We present here a structure-function analysis of one of the best-known HCMV immunevasins, UL16, and its interaction with a cellular ligand for NK cells, MICB. The normal function of MICB is to activate NK cells by engaging the most well-known NK receptor, NKG2D. HCMV-encoded glycoproteins UL16 and UL142 selectively prevent the surface expression of MICB, ULBP1 and ULBP2 (UL16) and MICA (UL142), respectively, through intracellular retention. UL16 is a heavily glycosylated 50 kDa type I transmembrane glycoprotein whose structure could not be predicted from its primary sequence.

In order to elucidate the structural basis for the ability of UL16 to engage highly diverse NKG2D ligands and to compare this promiscuous binding mode to that of NKG2D, we determined the structure of the UL16 ectodomain in complex with the α1α2-platform domain of MICB (MICBpf) at 1.8 Å resolution. In order to obtain soluble and homogeneously glycosylated protein for our structural and surface plasmon resonance (SPR) studies, we expressed the UL16 ectodomain in Chinese hamster ovary (CHO) Lec 3.2.8.1 cells. NK receptors binding to MHC class I or class I-like molecules belong to two structurally distinct families, the Ig superfamily and the C-type lectin superfamily. While NKG2D belongs to the latter group, our structural analysis shows that UL16 assumes an Ig-like fold. We find that UL16, which possesses no structural homology to NKG2D, nevertheless employs a NKG2D-like binding mode to interact with MICB. A set of five predominantly hydrophobic core residues on the UL16 surface precisely mimics a set of five equivalent residues in the central region of the interface used by the structurally unrelated immunoreceptor NKG2D to interact with its ligands. The “rigid adaptation” concept is furthermore supported by the finding that UL16 engages its ligands via a rigid β-sheet, which does not allow for much conformational flexibility. Our structure shows that substitution of Gln169 with arginine, which is present at this position in MICA, would lead to steric clashes with UL16 residues Met59 and Leu161 that would prevent binding. In the UL16-MICBpf complex, Ala162 faces towards Tyr125, a UL16 footprint residue. Taken together, these analyses suggest that some NKG2D ligands apparently bypass intracellular retention by UL16 through alteration of a small number of key residues at strategic locations of their potential UL16 binding interface. To the best of our knowledge, the structure presented here is the first structure of a viral immunoevasin in complex with a stimulatory NK receptor ligand as well as the first reported case of structural mimicry through convergent evolution of a human immunoreceptor by a viral immunoevasin.

>MEPHSLRYNLMVLSQDESVQSGFLAEGHLDGQPFLRYDRQKRRAKPQGQWAEDVLGAETWDTETEDLTENGQDLRRTLTHIKDQKGGLHSLQEIRVCEIHEDSSTRGSRHFYYNGELFLSQNLETQESTVPQSSRAQTLAMNVTNFWKEDAMKTKTHYRAMQADCLQKLQRYLKSGVAIRRTVPPMVNVTCSEVSEGNITVTCRASSFYPRNITLTWRQDGVSLSHNTQQWGDVLPDGNGTYQTWVATRIRQGEEQRFTCYMEHSGNHGTHPVPSGKVLVLQSQRTDFPYVSAAMPCFVIIIILCVPCCKKKTSAAEGP[2x];>VDLGSKSSNSTCRLNVTELASIHPGETWTLHGMCISICYYENVTEDEIIGVAFTWQHNESVVDLWLYQNDTVIRNFSDITTNILQDGLKMRTVPVTKLYTSRMVTNLTVGRYDCLRCENGTTKIIERLYVRLGSLYPRPPGSGLAKHPSVSADEELSA[2x]>TPPNAPVVTYSDIVNDLIIMQGTAEAKSQLIITDSEGNTYTLTVPDNGKWSMAIPYPSEGKFTITSVDAIGNRSDDVPLDIMKEVPVISLSPDSDSGTVGDNITRDKQPTFIIGNLESDVVVVQVDINGTVYNAEKNADGVWFFTPGTPLADGSYTISVIASDAAGNQKNSLPITVTIDSTLTVPEIALAAGEDNGASDSDNVTNHTQPKFTLQHIDADVTGVTVNVTHNGVTDIYQATQGADGWTFTPPAAWNDGNY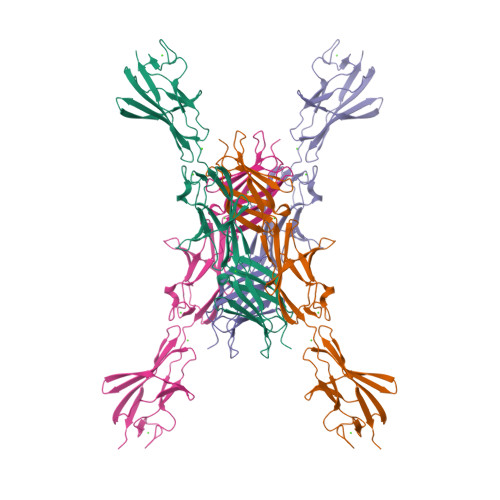TLSVTVVDRAGNSQQSASLAVTVDSTVTVT[2x]>[4x]MKVQYCDSLVIGGGLAGLRAAVATQQKGLSTIVLSLIPVKRSHSAAAQGGMQASLGNSKMSDGDNEDLHFMDTVKGSDWGCDQKVARMFVNTAPKAIRELAAWGVPWTRIHKGDRMAIINAQKTTITEEDFRHGLIHSRDFGGTKKWRTCYTADATGH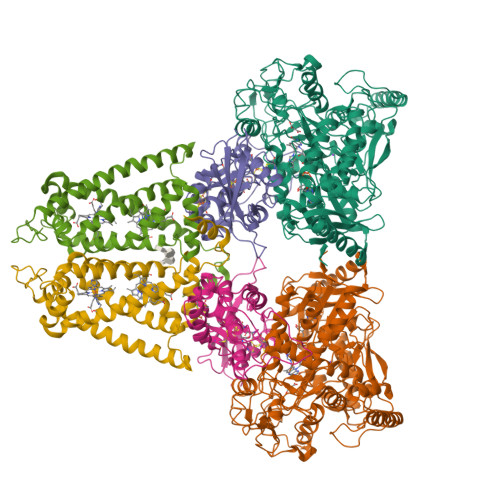TMLFAVANECLKLGVSIQDRKEAIALIHQDGKCYGAVVRDLVTGDIIAYVAKGTLIATGGYGRIYKNTTNAVVCEGTGTAIALETGIAQLGNMEAVQFHPTPLFPSGILLTEGCRGDGGILRDVDGHRFMPDYEPEKKELASRDVVSRRMIEHIRKGKGVQSPYGQHLWLDISILGRKHIETNLRDVQEICEYFAGIDPAEKWAPVLPMQHYSMGGIRTDYRGEAKLKGLFSAGEAACWDMHGFNRLGGNSVSEAVVAGMIVGEYFAEHCANTQVDLETKTLEKFVKGQEAYMKSLVESKGTEDVFKIKNRMKDVMDDNVGIFRDGPHLEKAVKELEELYKKSKNVGIKNKRLHANPELEEAYRVPMMLKVALCVAKGALDRTESRGAHNREDYPKRDDINWLNRTLASWPNPEQTLPTLEYEALDVNEMEIAPGYRGYGAKGNYIENPLSVKRQEEIDKIQSELEAAGKDRHAIQEALMPYELPAKYKARNERLGDK;>MGRMLTIRVFKYDPQSAVSKPHFQEYKIEEAPSMTIFIVLNMIRETYDPDLNFDFVCRAGICGSCGMMINGRPSLACRTLTKDFEDGVITLLPLPAFKLIKDLSVDTGNWFNGMSQRVESWIHAQKEHDISKLEERIEPEVAQEVFELDRCIECGCCIAACGTKIMREDFVGAAGLNRVVRFMIDPHDERTDEDYYELIGDDDGVFGCMTLLACHDVCPKNLPLQSKIAYLRRKMVSVN[4x];>MTNESILESYSGVTPERKKSRMPAKLDWWQSATGLFLGLFMIGHMFFVSTILLGDNVMLWVTKKFQLDFIFEGGKPIVVSFLAAFVFAVFIAHAFLAMRKFPINYRQYLTFKTHKDLMRHGDTTLWWIQAMTGFAMFFLGSVHLYIMMTQPQTIGPVSSSFRMVSEWMWPLYLVLLFAVELHGSVGLYRLAVKWGWFDGETPDKTRANLKKLKTLMSAFLIVLGLLTFGAYVKKGLEQTDPNIDYKYFDYKRTHHR[4x]> MG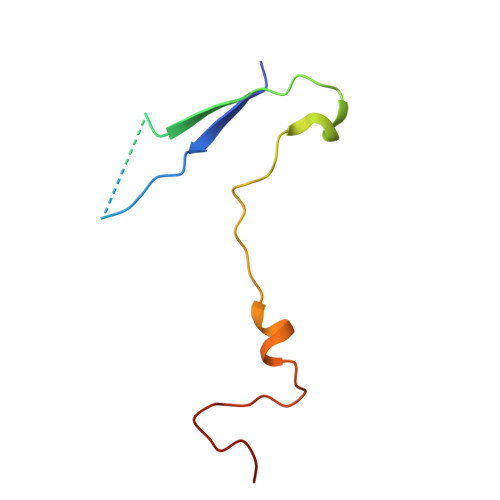AQVSTQKTGAHETGLNASGRSIIHYTNINYYKDAASNSANRQDFSQDPGKFTEPVKDIMVKSLPALN>[2x]GSHMAHSKHGL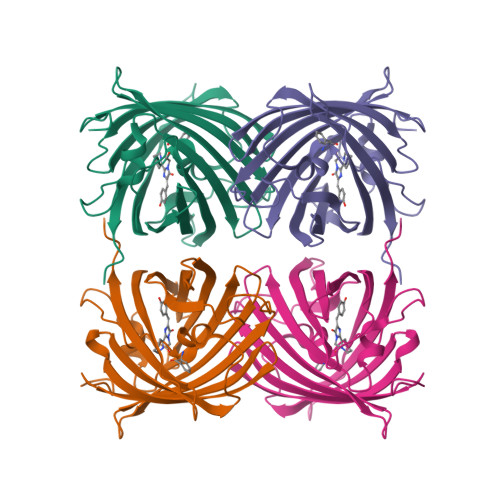KEEMTMKYHMEGCVNGHKFVITGEGIGYPFKGKQTINLCVIEGGPLPFSEDILSAGFKYGDRIFTEYPQDIVDYFKNSCPAGYTWGRSFLFEDGAVCICNVDITVSVKENCIYHKSIFNGVNFPADGPVMKKMTTNWEASCEKIMPVPKQGILKGDVSMYLLLKDGGRYRCQFDTVYKAKSVPSKMPEWHFIQHKLLREDRSDAKNQKWQLTEHAIAFPSALA> MSNAALATAPHALELDVHPVAGRIGAEIRGVKLSPDLDAATVEAIQAALVRHKVIFFRGQTH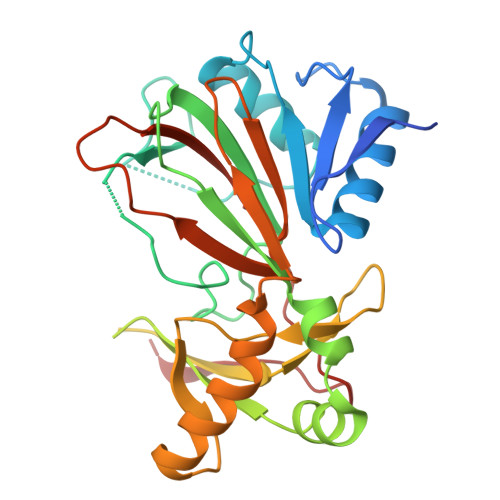LDDQSQEGFAKLLGEPVAHPTVPVVDGTRYLLQLDGAQGQRANSWHTDVTFVEAYPKASILRSVVAPASGGDTVWANTAAAYQELPEPLRELADKLWAVHSNEYDYASLKPDIDPAKLERHRKVFTSTVYETEHPVVRVHPISGERALQLGHFVKRIKGYSLADSQHLFAVLQGHVTRLENTVRWRWEAGDVAIWDNRATQHYAVDDYGTQPRIVRRVTLAGEVPVGVDGQLSRTTRKG Protein synthesis in mitochondria supports bioenergetics of eukaryotic cells and is executed by dedicated mitoribosomes. To provide a representative reference for studying protein synthesis in the mitochondria of fungi, and to reveal how the mitoribosome functions in coordination with its translation partners, we determined structures of the translating mitoribosome from the representative fungal model organism Neurospora crassa. The fungal mito-ribosome consists of 78 different proteins, 23S and 16S rRNAs. Forty-eight bacterial orthologs are extended, and 30 proteins are mitochondria-specific.

To further improve the local resolution, focused masked refinements were performed using the masks for the large subunit (mtLSU) core, central protuberance (CP), L1 stalk, uL10m region, the small subunit (mtSSU) head, body and tail. In the CP, we found an extra density in the pocket formed by mL40, uL5m, and rRNA H84-ES3. Based on the density, interactions and the abundance in mitochondria, we conclude that it is most likely to be NAD. Positively charged residues of mL40 and uL5m interact with the negatively charged NAD phosphates. The pyridine ring of the nicotinamide is held in place by π-stacking on the base pair of A2755 and U2759. Arg295 of mL40 forms π-stacking at the other side of the NAD pyridine. Therefore, NAD bridges the mitoribosomal proteins and the mt-rRNA at the core of CP. By masked refinement on L1 stalk, we improved the density that allowed building its complete model. We identified an additional protein component, namely mL108. The protein mL108 interacts with both the L1 stalk rRNA and the protein uL1m.

> MSNLFRSLASSMRALSLAAPRATAVNTTKTVVSTHQTRCLSQGLLSRHICTPMCSHNRPVAVCQSAKNGLQSKQQSRGMKVHSAIKKRCEHCKVVRRKANKRQNGYLYIICPANPRHKQRQGYR;> MSTCQQVARPLVRCLRQTGPGAATCSTRSVAVAAVRPFSSTPMRKEEGATTTTTTSPVDSTTTPPPLPSATEAKATVADTVVGGPELGSRRRRAALATTGNLPFEQLPYQCFQDARKILQQDRAAKIAQIVKETEKIKLIEARDASEFEGGEAAKQTRIKSLRKYIEELKILADINDPEVKRRFEDGRGDMTKPVYRFMAERRWRSMDYKIIAQRISQFHVVPDLLPAFDPTMDVKLSFRGYQVSPGAILDSRVTEVAPTLRMQVFDKGERLLTVVVIDSDVPDVTHDNFKRRCHFLAANIPWDPSKTVLSLRSVGDRVEGDVGKPWLPPFAQKGSPYHRLNVFVLEQKPGAKIDGEALKKHLENRENFSLKGFREKFDLEPVGFNLFRSEWDEGTAEVMERHGIPGAEVEFKRQKFASLKPPRKARGWEAKRQKPKYKSLWKYVKRIA;> MVSATKKPVSAMSAKNSTRHRKVSHKVTKTIATAKSQVISNKAMKIRTKSWKDMPSPKRRRRINAMVDELRLQGNVKMPKPGKSTYKAGGGERVRLVKAASTLPTPPLTPPVLSKPTGSASQSKGDLKPKRPTPEKKRSVSKRDVERFFLSTQTSTRRRENTPIHAPIMSSTFTSLRGLATRLFAGGARPSPSSLLLPNKPATAALPTAIQHQQTASYASKGKSGPPAGMFSGQKAGSKKSKGPKQVDPRIINILRHFAVLSPKRIPPPLRFGRNRYLRHWTIHRAWLLFRRQQREQRERILMQQHQSMSNACEELRNTEGPGTRETGYLYRVAMLKNGVYGLKSIPIEYASRALVETPGRQAWNHEWKR;> MQPTRILQGLKYRKLRLTTKDVNKGFYKGNRTGSMGTHTSYGTYKIDYTKVRTYVCPDLTGFKLTPFVSKTIRPVHDQFPGDKLGPKNPATYLARWKSENGLD;> MTVKALTQISSAGRNGVGAFVLQCKKLDIHYSDWAGSSRGMNGFIKSLLPKFAAANPQIEFVVSPRPAKHPILMGHYINGRTKAICVRNMEPLEILKKAELLRDASGEKPQKFKKPVTSTNPSVRGVWSPYHGQGMAV;> MKRIATPSLTSRLLVAARSGVSPATAAIRSRSAISVRSQSTAALAQHDASHDLNNDRFPPLEPLPPAAESLPSPLPERALTSAKLAALHARLNLSPKIPLQTLARTLVDASADENPQFNNANLAFVGQTLINYHIAEWLLCKYPRLPQGILFSAMKAYAGPKPLLQIARSWGVDTAAVPGGEVDPGLLQFDALKPGVAITNFGYKRTELAYLEKFKWRRGMASRVVLDDDFGDVVRSDPKVAADLEKAMEEQDQDKTPDEEEAEMVANEQDQDVSYDRYGNPDTRAAAERAHAYFVRAVVGAIYAHCGREAAKAFVKAHIMSRTLDIAKLFEFKYPTRELAALCAREDFEPPVARLLSETGRQSRTPVFVVGIYSGSDKLGEGAASSLDHARFKAAMNALKAWYLYSPGENPRVPSDMLEEGAKPWTPAYIDMGEVISR;> MSASSRGAALLRSQQRSICLQCRNQTRVLAPAGVTSAPRRFYSAEASATATATATATTTTTLPPPHPPVTTSTGTHAATSTSSQIYRIKSGVILTRPPLLTRDLTPFEESFYFYQKRLNERLTAPFRKDFYFKKDTAADLDWRIKLKERHGVPAKDIGRYNPRGRMAWNDEVLVGSQTSSRKHMVEKLLADAEMRVSEDGEEIPAEDRVPVEKPMPRRTEADEKGDVKRLDRALDKTLYLVVKKKADKEGEEAKWMFPTGVVPTDEGLHETAARILAESAGVNMNTWIVGRVPVAHHVVRPVFGQKDGALLKKGEKIFFLKGRIMAGQADLTDNLHDLVDFKWLTQEELRSTLAEEYFHSVKGMFAER;> MFRSTFFGLSRAIVQPATPLTVRAAFQSRFYSAAAAASQPTTTATTTTPLQQQQQQQPTTQPTTPIQTQTGAAPTESTKPVAKPYLVGRAWTQRLPVYHLAKRGGNKKLTQIKKVQGDGQALRRDLAQFLGLEVKEVRVKVPTGHLEVDGHRREEIVKFLDGLGF;> MRRIPRIPSTASALCSSSSSVASTSAAPLRTLRAAADSSSICQSCSFSTQTSATRNRVWQNTVQTQRRCASTVTETTPEAPVAAAAAETATESTETVEQQRKRKGGFFETQRQVNLVLPGQPTRADAPEKIRDPNYEPATSGAGLQEIGGMSDWWSKPEHFRDGGKQFEYQGFAPQEKITDPRLLKVILRRALAEGLALKKFGANPKNPADMASIIGNGDHWQRTVSVEMCRGENGELSLKNESDLQKVWILMRNAAEKTYYQREWQEEINRLRSLGEKEQAKQLLEEGKKLGYRLKSEEGSLVKLTVDEAVELRKSWNNDWKEAIIRDPVVKFYAAKRIQKMTGHILSDGKLTSIQTVANFMDALVTPPKPKKLAEQIEQSSILPELPNVKVYPRRVTPVDKERMVGRWKVIQKELQKRELPVLGTGNHGKYVELKWLGSKQ;> MAALTPSRSVFASTCKTIAQQCSRRPVAVQQLAAVPVARQVSSSSAVQQEQDASGTSSSQQPRPRWSYTPERMKGPGFSLNLVKDPRRKQWMVNSDPAKLDAFYDAFLGQGGSRMLSEETKWLAVTHKSFDYGRRGYNTRLAFLGRQIIALETTRSILTSPVLNEPIVDKYGRTPYNHAALANIDKLIYTQPLDIMDKTKIARMGIDFGLLTVMRWKPRMPEDLESSGVVVVLNSTLFAIIGAISLEKGAAVAQRIVREKILKRLGA;> MLQPQFRPLLAGTASFAQTVLGRTVARCYATKAATQSASSTSTSNTSKDAKAKIVTPYVRDAGMMRTYKPHTPGIRHLKRPINDHLWKGRPYLPLTFPKKGQSKGGRNHSGRVTVRHRGGGHKRRIRMVDFERWIPGPHTVLRIEYDPGRSAHIALVKEEATGRKSYIVAADGMRAGDVVQSYRSGLPQDLLDSMGGVVDPGILAARTCWRGNCLPVSMIPVGTQIYCVGSRPDGKAVFCRSAGTYATIISKEEETREDGTKVMTGKFVNVRLQSGEIRRVSKDACATVGIASNIMHHYRQLGKAGRSRWLNIRPTVRGLAMNANDHPHGGGRGKSKGNRHPVSPWGTPAKGGYKTRRKSNVNKWVVTPRVRNMGVRRNKKTT;> MAPRLPARCWRQLSLVERSATHTTTTAAASSLLLAGRTTPTFSASSPSTVFPSLLPQITKRGVKYGWSTLPKRSRPTRFNQVTQGLPAPTSGPAAALKRREKTTPLRTGVLAVKKGMTVFMGRTGARIPCTVLQLDRVQVVANKTRAKNGYWAVQVGLGERRAENVGAPQLGYYEAKGIPPKQTLAEFKVRNQDGLLPVGVQLFPDWFHVGQVVDVRGITRGMGFAGGMKRHGFAGQEASHGNSLNHRTIGSVGGSQGSGSRVLPGKKMPGRMGAQQHTVQNLPILMVDNELGIVVVKGAVAGHKGAVVKVQDAVKKAPPPEEFVEATKQLLNERFPDAEEKLQAARKLHLELKEARRQGLIDSLIKNGLTEKADGNAAVEASA;> MAGKGLKSLNEAMNALSIASKSCRALPMRQSSILPCRRSMASVATPPAANITRSVSEPWQPITNVPVTVYSFPELEPRSLESYSARHLHLPLRRDILHLAVIYEGDSTRRGMASTKTRYEVHGSHKKMSPQKGTGNARRGTRQSPLMKGGGKTFGPKPRDFSTKLNKKVYDLAWRTALSYRYKRGELIVTEDGLDLPLPNDFLWLAGGGKLSRELEDGYVRKWVHEFMTSLNWGKEAGRTTFITGDKRPNLFTGFELAGAEGRALELWDVDVKDLLETGRIVIERSALKEMIEDHQSDLVTRVAVQGLRQKGPNLGEVLVRAPRY;> MASLRGVSRSARALQPFSAQFAVRRCASTQTGAGAAAATPKSNIPDLAELETRSALDAPIPSEEDKKEFRPWKRAADRKARLPSSRYQYHPPKYNRGPLHPIQSPPSSDPIARDFVPGPFNMPRLKETFRTVMASDLMTLAYIHTPPGTPKKEPTERLRAWEGDSPYFANRARRAPRGAPELPIRERDISFRNIPEIKEITVSTFVPLGLKNPDLLIVARAVLLAMTGTMPEMTRSKNNVVQWQLQANKPAGCKTTIYGNAAWEFMDRLIHLVLPRIKDWKGVPASTGDGSGNVQFGLNPEDVQLFPEVECNYDMYPAKMIPGCHIAIKTTATSDRQAKLLLQSLGVPFYSN;> MFAPSRRRVLEAVASSSSSPVVTLPGFLVPAFQQTAGAAARRNFSATTTRPSKLGRTPLSIPPGVEITIGEPFVKRDMTQWKQQPKRKITVQGPLGQLEMDIPDFIKIDHDAEARRATLSVANRDEKEQREMWGTTWAYLNRFIMGVSEGHTAVLRLVGIGYRATIDTRPEKEEYPGQQFVCLKLGFSHPVEMGVPKGMKASTPQPTRILLEGINREQVMTFAADIRRWRVPEPYKGKGIFVNGETIKLKQKKIK;> MTASALSKWPTCLACLRRLAQPFGTSAARHGEPRARAVPVIRPIVHTQTRAASHRMRLQDQGVVVRLLEDIPKFGRKHAIFRIERGRMRNEWFPKNKAEYMTPARFQELGLTRDAIGEVDRSFVIMSALEAATRPKPEEQKTEEPVPEVQISQVNVPDVTPETAHALLSELIPNTLTFHREPVPIPISQPKPALEPKISPLIARHVPASTPETPSTGEARRAIFGSVSSSDILNQIKALVSGHEEASRIVLGPSSVKIVGLAEDNDRIRHLGRWEIEIAVARAGGLDPVRKSVEILPSAQ;> MSQTVGATRLAYSRVWHHISAVTPHPTLSTIKAPSEAITPPSLGRLASRIATILMGKHKPIWDPSTDCGDYVVVTNCAGLYTTGHKKWRKTYYRHNTRPGSLQAITMDALMEKHGGAEVLRKAVSGMLPKNRLRDKRLARLKAFEGDAHPYKENLVRFGGKVVGAPGWEEAVKAIREADMERL;> MIQLKTMLNCIDNSGAALVECAMVVGQKRHASIGDRIVVVVQKQRGADSAGMAASSAATKVKRGDIRHAVVVRTKQKVQRRDGSVVRFDDNACVLINKAGDPIGSRINGVVGQELRKKKWSKILSMAPMQA;> MPPRLPLAQAARCCQASLTARPSVPASSPTSSLISLFAALSVQTRSASILASLSDNRGAYHKRIRKGRGPSSGYGKTAGRGTKGQKAHGHVKPWFQGGQTPLIVSHGRKGFVNQFAADMSELNLEKLQEWIEAGRIDPTKPITPKEIIKSGIIGSSIKDGIKLLGRGKESFKIPVTITVSRASASAIEAIEAAGGKIVTRFYTKESLKRLVEGKSLHTDKPLPVGKEHVEEILAQARSLKKKYYRLPDPTSRWDIEYYRDPAHRGYLSHQLAPGESPSLYFKVPTGGEKVKVVRADKVKASKTGDVASEKLF;> MKHNASSALLSAFQGLRISSSATPFRAASLATSAVRRPIAPTPVSVASHVRLFSATAIQAGSWLEPNLNRKKKMMKGRPRVPTGGSTKGTTVVWGDYGLRMRDHHRRISAQQLKLAEDTIKQRLRGQKYRLYKRVACNVGVYVSGNEMRMGKGKGSFDHWATRVAVNQIIFEIRGQLHEQVIRDAFRLAGHKLPGLYEFVKKGDPPVVGITKLEDGLTVEDLKNPRKKLLMPEITQSAASTSSTAAPPS;> MAGAHVKYRHLSRSSAHRQALLRNLVTSLIKNETIHTTYPKAKEAQRLAEKLITLSKRDTETARRSAQGILYTPDQLLPKLFGEIRERYANRPGGYTRVLRTEPKDQYSQAPSAILELVDGPKDMRFAMTAATVARDREQKTESTDLTKKNMDKVTRFRKDGMRAFEDMVASLRDMKFTAGAINPKEWKKLDR;> MNVTASLSRRPLGCLKAGLCQSLIRGYATAVAASTTQSTGALPDHNFFRIADKHTKKTRTAFAVFTPPKSPTTLPPSSVVTKSKAFKIANSKLPPLMTKPPSDPMPLLTQQQIARMDPTGARTALFSKARHAARVGDVLMVTHRRGGEPFAGVCLAIRRSGIDTAILLRNHLGKVGVEMWYKIYNKNVAGIEIIKRRAKRARRAKLMYMRQPKHDMGSVEQYVFAWKKMRKVLSSKGLTGGVGGGGGKQKGQESKKKN;> MSRALLRSVLELRTPVTRLPPSFLLPFRPAARFLHQTAQQVEPTSQSDAAAAAATLLKASPPKVTTATTPEAPAAVPTSTPFSQQPPISQQVKELLPVLAAQPGHYTTIHIHGKPYLVTEGDTVKLPFKMPGVAPGDVLRLNRASVIGSRDLTLQGAPYVDERLFECRAIVMGTESEPMRVMIKKKRRCRKKKHVFSKHKYTVLRINQLKINDVSSL;> MSLNVPSRRLLKSAPSSANALVPALQSLSINTRSIHTTPSQQWSLFGWGKQKVEERNKVKEELKQSELARTRKPTQEEIFERVRGRLEGDSIFADTTPSSQLAAEQDKHKDWATASAEKKLAAAHAKDQTPTGISLKKDHLVRVVDPDPRSRVRWERKMVIRKLQRGTDPWSVEPKAERIARTERKLVYKTGYLPTSVKKLVHLSRQIRGKTVSEALVQMQFSKKKMAKEVKTELLRAEAKAIVTRGMGLGKAAAAAAQKETGAEPVKIQTKDGKHLEIRDPTRIYVAETFVNKGFTRGVELDYRARGRVFKMNKPTTTMTVVLKEEKTRIREHQERVAKKLRQGPWVHLPDRPVTSQRQFYSW;> MASVAKTGAEALRNAPFRVGKKQIFLPNHVITFVRPLPKQPPNLATFIVPLEFNKLDLRDYLYHVYNVEVTGVRSFVNQRMHEQRHGDVGNWRRPKSQKMMIAELAKPFVWPKPPAEDAREAFDYAMWKKQKTAQEQDTKFQGIRAQGEVVPPSQFEVTKDRKAIKARQSKFLSGEETWAPGKVNAFLNSKIVPEEEGWSEVEENLPLDESAESAAEESSSKGSETRQ;> MDKLLRRVRMAEGMVARRAQRKNALLKRITERKQNKKNGEAFTEAIQQRKAAVEARNEDWMLGPLAPRRELDEITLSNGNFFGSLSPTRALLESEVSEEERKARVAWCGSPKFLCIAPGDRVVVIEGHHKDLIGTIEKLNTRNMTVEIQSEKLKTNTTVPQFMQNDADKPVTQIYARLPISSVRLVHPLKDPQTGEYRDVIIRELRPRNIVHDRPTRTRSMRRFVPGENIIIPWPKQEPIKREDQPADTLRIDVDEKTFVPTLFRPPAPQQVLDELRNKYSIFRTRHTPEYIAKKEQEEQEKEAKKSAAKAMLTPVQEYNRKQRELRRARGQPALTEEMLAKIGEVVARNKLGHHQAPKVKEETVAQIEKAVEQLSLGGGQEDAATTTSPEQPKVV;> MHLAQLRQPLTRAAANSCHSVCRLPTTHSSVSATAILSEQFAHLRIGPSSSNVAVEGRRYASVKAQGAYRLKPKRTIPKKLGAKKTGDQYVIPGNIIYKQRGTLWHPGENTIMGRDHTIHAAVAGYVKYYRDPQLHPDRQYIGVVFNRNDKLPYPKDAPRKRKLGLVAVPRKVEEVEKPTMSASGLPLFVTRHETIEIPPPAVTTPAAAGKAVKGQGARVSASGAAAVPASSSTISASASSNSNNGGSSVIAELIKEKLAARAEYNARQSALRKLQQQKMLARRGTRVLRLMNNYSYRETNWEIGRLIGDPGSVPGTEKVGSRKAKFRARRRRRNTFLLGIKERKLAKADRREEYRRRVREKREQRLVQRKEFLAKQREAKKAREGGAAAEKSEKKEVKAEKPAAAAPKVEKPKAPEAAKKESKPKVEEKKAAAAEPKKDSKTEKKD;> MSSFLVRPFCLRATTTTTTTTTTTALVQQQLRALTTTTALTYHQPRVPSSAIPIPNVSGRVPLPDSTPVPEDFKIEIPSYPYGPRRVYHQSNTGLYGSALIRFGNNVSKRNEIKTRRKWRPNVQQKRLWSKSLGVFVRTRVTTRVLRTIDKVGGLDEYLLGHKAARVKELGPWGWMLRWRIMQTPEIRERFAKEREALGLPPRREEDEEKSLEEQLREFQVAGIQFAEGKAPKTKGQLKEEADRLIKKSETEEFGLGQEEDLFMKEEPKPTKMA;> MASPAALRPSMGAIMQTCRSAATAPKVAVAVPVRALSTSAALLKRHKYPTARVTRDNSKQRGESALRKSGTRWKLSVSDEPLPEPVPREELPPIQVDENHGLWDFFYDRETVAMAPLEHTKHGRAWTVSELRKKSWDDLHRLWWVCVKERNRIATANWERTKSELGFGLAEANERDRNVKQTMRGIKHVLTERFYAWEDAVKLAEQDPEIDLSNPENPYTPSTFLEAEETAEGAEASETQSTTTEIDPTTIPSSKSQAEAPRV;> MSFFRITLHRSAIGLPKRTHGVLAALGLRRRNQTVFHPVEPQFAGMLMKVKELVRVEEVPHRLTKRELKDERKPDAGFVVEKQVRRFIPGVGVQDEVDFSKVVEELKAQKVENVEGVEKMVVEGGAVVRDGKRAGDLGVRTRSDWEVIGKMKSVLPKVKAL;> MSSKLPTTLLRRPSALPSTTTYTAYSASRPTPPSCTAHGAQGQQIRNATFVPRHRRPYQFTQLVQLSDGSTFTVRTTMPTALYKSAKDSRNHLLWQPSDKSLKNVELDEAGKLAAFRERYGRGWDLDAKMTPEEEAAAAAALAAGGGAGVPGGKAAKKAAEEALLAKKKKEEEEAAKKAAEAEEADPFDSLTDLISGYATENMNPGLNFKETRHYGKKK;> MAAMTAAAAAPAMRLFNPSTFFQTLRTQRFGVPALNFAVPAAAISLLPSIPSLLEDIWEGILRAVPKKKTSHMKKRHRQMAGKALKDVTHLNRCPACGNLKRMHHLCSTCLGKLKGFMDRNGGSNAKAY;> MAKKAKSRIINVRLISMAMTGYFYTFTRPRTSLPMSMLKYDPIVRRKVLFLEQKRKGRS;> MSRIFSSALQAVFKPSAFLPKTATRSFSILPSLRPATLSSTPSTIFRAPNAITAPSASPSATTGIDGEVLDLLSASSLISSHPALSGLGSQIRCGPRPTMSGATRLVQKRRHGFLSRVKTKNGQKTLKRRLAKGRLRLSA;> MEASLSLFRPVATCCRRVALSSSSSSSQKAAAVAGISVRYQSTANRTKRMLNIPPHESFLNVPVEGDRIIFNPPSSEASVYHTPFKFLPRSDPRRRANIYKLFKPPQAPITTPESSSTDAAAADQHGDLPPVLYNPTKSYNVTPEQVEEIRELRAKDPKKYSVTYLSNKYNCTKVFIMMCTQAPREHQEQHKLARARTAENWGPRRAAAKLDARRRKEMLHRGEI;> AATVKQHVQLALSLPPRLRTFLARYPPASILPAGADPETHKTPYQEESPNPFMPTKHPITGKWHNPKYSLRRQAELVKLAQEHGVEELLPFTRKLNEEKLRKRVELGLRVKGTGVGEKVKGHKHERTLVAKMEKRREAMLAMPDLIREWKKVGKRNWTKFPK;> MFGAFRFTNPLSGGLLWKIPWRMSKFQKLRQRRRLRAVDNVVATIENALAKKGETVKAVERWRAEMPTEAEMLPKDKYTIFDRKEKRYRKGIHKLPKWTRVSQRVNPPGY;> MNSVTTSTIGRLAFGVSRLSAVTNVAGAVRHASTHPTTAIPKPTTAVLKTSPLAEETAVELKSPSRLQLKSEPGNKGNPKGHGDRIWAFHHIEQGQVIYSTKPVISHQHLIRQQPFTGKNLVPRKIRKDYWRPLAMIELAGKDQGAVGRSVYQKLREFKKRHELDWANEAEEGRKLMHKSKRERGQELNDQKPNSVADMAAVLAGAGKGNLMWQVSRLGSSSELVGEIKKASGAVEKGAVVDVKRQLRRATVYWTNEQDKFHAREWSDNVSHEVGIPGEAEKKRMPIRMSSE;> MASTQQCLASLARLSLSTPTRAALPTIPKFLVPSVAASQVRYATNNPNKGGAKKAPKKKKQYKFFKSWDLTGQQQFSLCDAMRYLRAVEVGQPPLSVKYEVHVKLRTKKNGPVVRDRVRLPTPVKTDTRIAVICPEGSALQEEAKNLGAVMAGEETLFEAIRSGNFPFNKLLCHTESEGALRKANVGKLLGPKGLMPSGKTKTITNNLEATFRDMIGMDEYRERNGVVRMAVGQLGFTPKQLAENIRVFMAKIKSDIGKLDDTTPKMVEEVVLSTTHGPGMSLNAEFAPTDDKIKPEDLESVM;> MSLRLSRPAVRGLGSAIKSSRISSRSAALLVPSTSTSAFSTASPQRAAAAGHLRLPDDYVPPTQPPSARPVDTRKSQLLRTYTSMLRSTPLMLIFQHNNLTAIEWAAIRRELSLALSNVPVPEGAPDITSKIHLQVVRTRIFDVALKTVEFFDPSTVEPTTATTATGTKVPATYNHDLSKHAWKAVKEATKNTEAVEKTVYGQLAPLLVGPVAILTLPSVSPAHLGAALSVLAPSPPAFPAPSRKKNPGYYDLTCQSGLQKLLLVGGRIEGKAFDYDGIKWVGGIENGIEGLRAQLVHMLQSAGMGLTSVLEGAGKSLWLTMESRRSVLEEEQNPKKEGEGEEEKKE;> MSKAAKGGAGGVEQVVKLIVGAGQASPSPPVGPALGSKGIKSMDFCKEFNARTAHINTGTPMPVRVTVRPDRSFHFDVRTPHTSWLLLNAAEAPIGKGGKRKGASNPGKEVVGTVSLKHVYEIAKIKQSELRLSGLPLEGLCRAVIYQARSIGINVIP;> MLTRFITDVSTRFNPFSAKAKAARLFLSFLPPNARSNGMNITTQLLPRNSTETPLLYVKFKDGKEMNLDVENMGIKSIVEEVDRHSRILQKQADLNDG;> MICRTCLRRASGFARPAAAAATRPMVAASSRAAFSTTFSVCTPPAATPAAAAPATSTAEAGLAPVPGAATTEQAKAAISSCPAGTKLNGLNYFKNKADPVALPDEEYPEWLWRCLEVQKKTDDAADADAGDEFSKSKKQRRLAMKRARAQEAKILASGDLEALAPKIPLQKQSVNLPGAVNGGVQDAVLADEKREELRKAMRKERKAKIKESNYLKAM;> MVGVIRRLNVVRELLNIRAGPGAALLPKEVTKVHMQFAHRIEEGHMGPRKFWRENLPKLKYWNPAVPMVINRTTDQKGPAVMTIYFRDDKDAKPSSTPFPTSSADGSSPAPKPAQGERIVTIDMKNRNSSVILKEFLDKTGAVAVQPTAKDEEEFREFEDLHRRSEIDRERIRKMNDAKKREKAMLAKAMSDAQSIKAASA>AVINHDAVPVWPQPEPADATQALAVRFKPQLDVVNGCQPYPAVDPQGNTSGGLKPSGSQAAACRDMSKAQVYSRSGTYNGYYAIMYSWYMPKDSPSTGIGHRHDWENVVVWLDNAASANIVALSASAHSGYKKSFPADKSYLDGITAKISYKSTWPLDHELGFTTSAGKQQPLIQWEQMTQAAR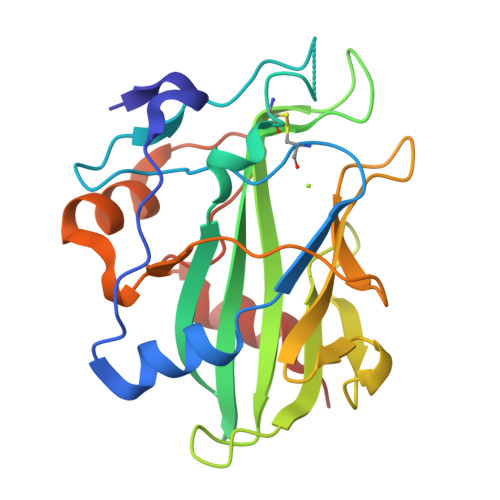DALESTDFGNANVPFKSNFQDKLVKAFFQHHHHHH[4x]> GSVPALWSEVNRYGQNGDFTRALKTVNKILQINKDDVTALHCKVVCLIQNGSFKEALNVINTHTKVLANNSLSFEKAY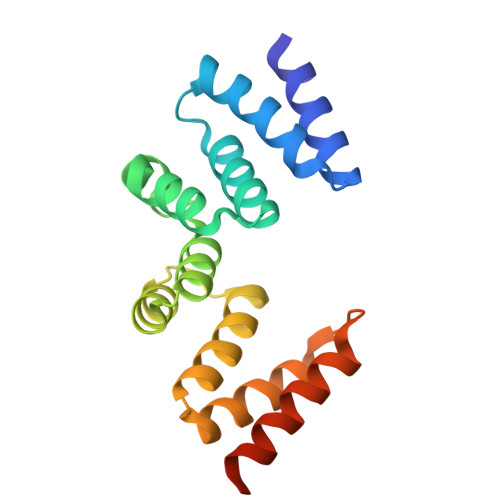CEYRLNRIENALKTIESANQQTDKLKELYGQVLYRLERYDECLAVYRDLVRNSQDDYDEERKTNLSAVVAAQSNWEKVVPGS> QLY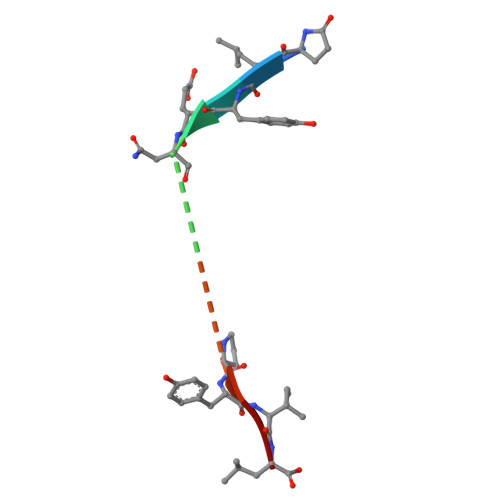ENKPRRPYIL NAPHTHALEN-1-YL-ACETIC 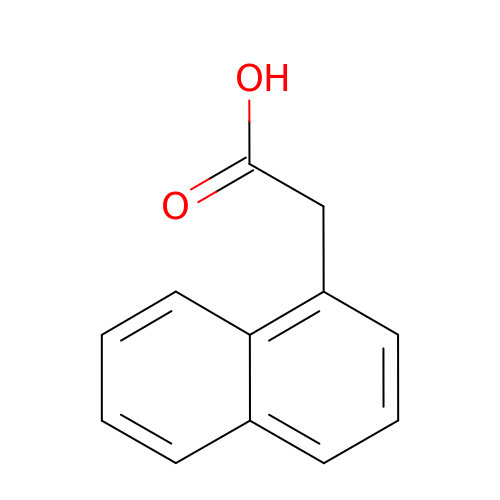ACID | C12 H10 O2 | PRPINYUDVPFIRX-UHFFFAOYSA-N> MEIDELTALGGLLHDIGKPVQRAGLYSGDHSTQGARFLRDLAENTGRAEYELLSLFSEFHHKGHMKNDELMIRRIKELSPERFGLTMEDVLNALWIVYEADNLASGEREEGQPQASRPLYSVFNPGKAYPWAELDFEKELPVPGDVFSIRSQDYRELVKRLWEELSKAKLRSDRLLPVLEKYLTFVSSVTSEGNIISLYDHMRMTSAIALAMLRAGCTAEDVRSGRCRKEKRFLLIEGDFSGIQDFIYRVSGKGTLKYLRARSAYLELIGWDVVLEILSRLGLTRANVVFNAGGHFMIIAQNTPDAVKELEEIRAKAVEWLYREFESDLYLAIEWEPVSGREFGREGGKNLFAEARKRLKHKLTVRKLKRFGEIKGLFEHGHTERLAECPVCGRELPEGKLEPSASDPETKVCPTCNRLVSLGGNLPKLLGFGRTAKNDAGVLVEGPFSGFVPYLQGGRPVGEQILVKNTLNPGEIPESAQFVPYFVADYFKKDPKGGVATFEELSMASTGTRRLGVMKGDVDRLGEFFSSMDSPSKLATASRFMDYFFKGYIGAIIEGKFGYIIGDVPSLRDWPEEPDIVVVYAGGDDFFIVGAWDQIFELAFRVRRAFNAYTGGKLTLSVGLGYFDERTPIYRMADVVSERLDTAKDEGRNRVFVVGRSRPLDGKHKLSYEWNHYEELWRTYAPRIYAGNGRLKGKLESKKGLLWKLLEIRELYVRDPNDVRWAYLTAYLLGRHGLSDLFPELVGIDTKAVERKEPQPVYWVDGVLKIVLMAVRR;> MHHHHHHVIFVAYHQKHGGYGRGGYGRQDRPQVDASRLFGESPDVVGIKKMLEGKGKQWEAIQPYFDNVVREAKNFLEWSPNKRLANAVTVAAYLTSQGLKTNQVRKILDMARTTELKVKRGEGDIKDDLVKMRYLLAYTVGKATGQSKYSLDAFHRILDPMLEVLMGSPKKENFEKFYDFLQAVV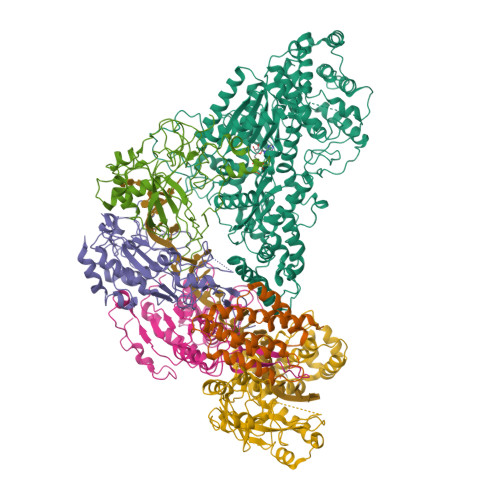AYHKFFGGGD;>[2x]MDRRFYGKIVIKGKIKAVTGLHIGSQRDISEIGGIDNPVIKDPHTGLPYIPGSSLKGRLRSLFEILVNSRLGEWREKYPSLANYSPGSCRPDNQENCGKFFNRKINRGWIHVCPDYETALACPVCRLFGASGKESNFPSRIIVRDAFLTKEWEEKWRAGEAITEAKIEVGIDRVTSQANPRTNERVVAGAEFEFEIIYNVENTTHWRDDIKNLLTAMALLEDSYLGGSGSRGYGKVKFIFDSFEFRPLDYYRTGKDEDIVSIDAREKSVSDILSGFDSLFSEVEGKLEAG;> MPKFIAVKLIPKGPFRDIPRADTLFGAIGNAISAIHGQSAVEELVDAFVGGARISSAFPYSGDTYYLPKPLSVEPALEGILTGLDEEERYTTAKRLRKAKYLDLKNFELALRLRPFTIPEEIPYARVDVPRVVLDRVTQDSSIYFWEEIRFREKSGVYFLYSGPREVFDGYIAPAMRFLGDTGIGGKSTWGAGLFEVEFHEMKIDAPGSEYSVTLSNALPTKTPVLWRLLRKGGWSFGRRKPRMTFIAEGSIVKNDPGGMERLELGLSHEVYVYGLTFPLGVELPEGLE;> MTERTLKVLSPLHIGTGNELTPVDIYPRENIIHVLDTERLVNDLMNLGVELNEILALLKNPPGDAYIWKGYIEEFHLDPSDYSIYTLKIHGKIGRKSMQIKEFIKLNGRPYIPGSSLKGAIRTAVLYKALKECGDARAVMRVVSKVNGDVARDIGRSEDVLDYYMSFLSRARIDRKRADDLLEAIVFGMEPDRRSKIRYEPKRDPMKALIVRDSKPVGRKHLAVYHVEVIGNPQPIPIWVEAIEPGAATDVEIHVDTEALRLNADYFNGLLWECLKERGEPGEVFEDFLWEAVDEFYTAVMKYETIEVQKFGRYTSQVRSFYASLEDHSGHVLRLGWGSGWLAMTIGLLLVEKGYKWENVRKKLGLGKKPGGSGFSREFPKTRRLADGMPMGWVVLE2-{[(4-chlorophenyl)methyl]sulfanyl}-7-methyl-N-(prop-2-en-1-yl)-7,8-dihydropyrido[4',3':4,5]thieno[2,3-d]pyrimidin-4-amine 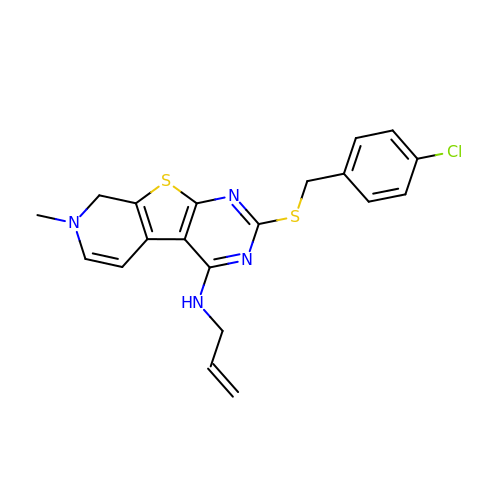| C20 H19 Cl N4 S2 | BXZWDXRSYVMRMU-UHFFFAOYSA-N>GMGIHQYFQSLSDLENIYRCPGKFKYQEHSVAEHSYKVTSIAQFFGAVEEDAGNEVNWRALYEKALNHDYSELFIGDIKTPVKYATTELREMLSEVEESMTKNFISREIPATFQPIYRHLLKEGKDSTLEGKILAISDKVDLLYESFGEIQKGNPENIFVEIYSEALATIYEYREMASVKYFLKEILPDMLAE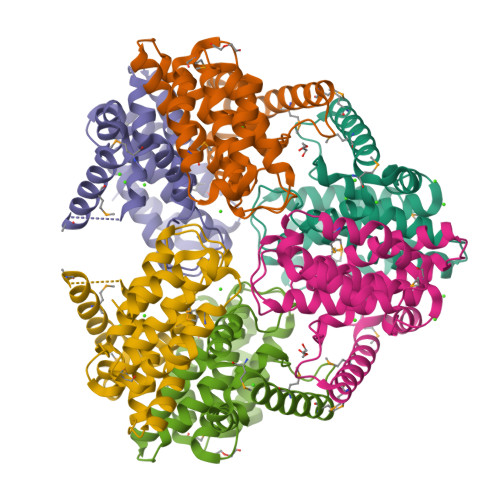KGIEKTELPQLTTEITTKALRDE[3x]> ASMKQPVVVIGSGLAGLTTSNRLISKYRIPVVLLDKAASIGGNSIKASSGINGAHTDTQQNLKVMDTPELFLKDTLHSAKGRGVPSLMDKLTKESKSAIRWLQTEFDLKLDLLAQLGGHSVPRTHRSSGKLPPGFEIVQALSKKLKDISSKDSNLVQIMLNSEVVDIELDNQGHVTGVVYMDENGNRKIMKSHHVVFCSGGFGYSKEMLKEYSPNLIHLPTTNGKQTTGDGQKILSKLGAELIDMDQVQVHPTGFIDPNDRENNWKFLAAEALRGLGGILLHPTTGRRFTNELSTRDTVTMEIQSKCPKNDNRALLVMSDKVYENYTNNINFYMSKNLIKKVSINDLIRQYDLQTTASELVTELKSYSDVNTKDTFDRPLIINAFDKDISTESTVYVGEVTPVVHFTMGGVKINEKSQVIKKNSESVLSNGIFAAGEVSGGVHGANRLGGSSLLECVVFGKTAADNIAKLY

Fumarate reductase is a flavoprotein enzyme containing the cofactor flavin adenine dinucleotide (FAD) that is responsible for reducing fumarate to succinate. Two soluble fumarate reductases, Frd1 and Osm1, which are essential for anaerobic growth, have been identified in Saccharomyces cerevisiae. Interestingly, a sequence comparison within the Fcc3 family has suggested that both Osm1 and Frd1 contain only a flavin domain and a clamp domain, and thus lack the cytochrome domain, which is critical for electron transfer. In the current study, we provide two structures for Osm1: one in a complex with its cofactor (FAD) and substrate (fumarate), and another in a complex with its cofactor FAD, substrate, and a second unexpected FAD molecule located in a newly defined second FAD-binding pocket.

In order to test the first hypothesis, we added an excess amount of FAD right before crystallization. The crystal we obtained diffracted to 1.75 Å and the structure was solved by molecular replacement. The shape of the electron density map appeared to be similar to flavin mononucleotide (FMN), showing a clear isoalloxazine ring and one phosphate group. The adenine nucleotide moiety of FAD, which was not anchored in this second flavin-binding pocket, could not be detected in the electron density map due to its flexibility. The second FAD-binding pocket was well defined, possessing a deep cavity containing enough space to accommodate the isoalloxazine ring from FAD. Six amino acid residues, including W295, F297, L298, N359, F362, and Y363, from the clamp domain and three amino acid residues, including K76, S78, and P162, from the flavin domain of Osm1 formed the binding pocket of the isoalloxazine ring from FAD. Among these nine residues, P162, W295, F297, F362, and Y363 directly interact with FAD via hydrophobic interactions, whereas L298 forms a hydrogen bond with FAD using a nitrogen from the main chain. With respect to the catalytic mechanism, FAD bound in the second FAD-binding pocket may directly transfer electrons to cofactor FAD because of the lack of a barrier between the two FAD molecules. Moreover, the edge-to-edge distance between cofactor FAD and the second FAD molecule was around 4 Å, sufficiently close enough for direct electron transfer. Taken together, we confirmed that Osm1 can oxidize free riboflavin molecules by accommodating them in the second FAD-binding pocket, which allows electron transfer between cofactor FAD and free FADH2.N-Acyl homoserine lactonases (AHL-lactonases) have important functions in decreasing pathogenicity by degrading AHLs. Unlike most AHL-lactonases, AidH is proposed to be a member of the α/β-hydrolase fold family. AidH contains a substrate-binding tunnel between the core domain and the cap domain. Taken together, the present results reveal the catalytic mechanism of the metal-independent AHL-lactonase, which is a typical acid–base covalent catalysis.

We further determined the crystal structure of the inactive mutant AidHS102G in complex with C6-HSL (AidHS102G–C6-HSL). Conforming to our predictions, the catalytic triad mutations S102G and H248G disabled AidH from degrading AHLs. Furthermore, in the structure of the complex of AidH and its substrate C6-HSL, each AidH molecule binds one substrate molecule in the active site. The carbonyl O atom in the C6-HSL lactone ring forms hydrogen bonds to the backbones of Asn33 and Leu103, and the Oδ1 atom interacts with the hydroxyl O atom of Tyr160 via a hydrogen bond. To evaluate the role of the nucleophile Ser102 of the catalytic triad in substrate binding, we modelled a hydroxyl group on the side chain of the mutated Gly102 according to the conformation of Ser102 in wild-type AidH. The hydroxyl O atom of Ser102 forms hydrogen bonds to the carbonyl O atom of the lactone ring of the substrate and the N atom of the acyl chain of the substrate with lengths of 2.89 and 2.67 Å, respectively. The distance between the hydroxyl O atom of Ser102 and the carbonyl C atom of the C6-HSL lactone ring (2.52 Å) suggests that this C atom is likely to be the target when the nucleophile Ser102 attacks the substrate. One water molecule, W1, close to the lactone ring of the substrate is present in the structure of the AidH–substrate complex. The entrance to the substrate-binding tunnel is in the open state upon substrate or product binding.

>[2x]MTINYHELETSHGRIAVRESEGEGAPLLMIHGNSSSGAIFAPQLEGEIGKKWRVIAPDLPGHGKSTDAIDPDRSYSMEGYADAMTEVMQQLGIADAVVFGWGLGGHIGIEMIARYPEMRGLMITGTPPVAREEVGQGFKSGPDMALAGQEIFSERDVESYARSTCGEPFEASLLDIVARTDGRARRIMFEKFGSGTGGNQRDIVAEAQLPIAVVNGRDEPFVELDFVSKVKFGNLWEGKTHVIDNAGHAPFREAPAEFDAYLARFIRDCTQLEHHHHHH> GSHMEAVQNRIVEAAERVPGVRGVIHLRARYVGQDIWANMIIG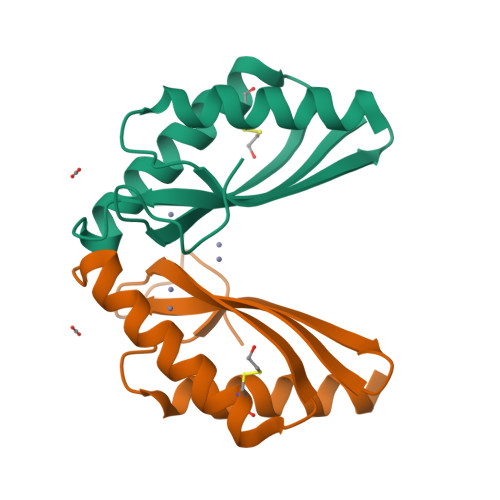VDPENTVEQAHEICEAVQAAVCGKIRRIESLHVSAEAREIGDTTKPSFSDQPLSFDEVMLSKVDN The large superfamily of labdane-related diterpenoids is defined by the cyclization of linear geranylgeranyl pyrophosphate (GGPP), catalyzed by copalyl diphosphate synthases (CPSs) to form the basic decalin core, the copalyl diphosphates (CPPs). Here, we used X-ray crystallography and cryo-EM methods to describe different oligomeric structures of a syn-copalyl diphosphate synthase from Oryza sativa (OsCyc1), and provided a cryo-EM structure of OsCyc1D367A mutant in complex with the substrate GGPP. The structure of monomer OsCyc1 consists of an αβγ domain and a catalytic center located between the β and γ domains. OsCyc1 catalyzes GGPP to form syn-CPP, in which new bonds form between C6 and C11, as well as between C10 and C15.

To investigate the substrate binding mode, GGPP was incubated with OsCyc1D367A before cryo-EM sample preparation. We solved the cryo-EM structure of the OsCyc1D367A mutant in complex with substrate GGPP at a resolution of 4 Å. As exemplified by hexamer protomer B, GGPP harbors a continuous and clear density in the active site. We found that while the overall architecture of OsCyc1D367A is similar to that of wild-type OsCyc1, a number of differences exist around the active site, mainly in the loop near residue N405 and helix α7. In the OsCyc1D367A structure, the α7 helix and loops near residues D192 and N405 embrace GGPP more compactly. In the structure of OsCyc1, K233, N405 and K453 interacts with the pyrophosphate, while M194 and E199 are close to the pyrophosphate of GGPP. In OsCyc1D367A structure, the DXDD motif and the conserved basic amino acid, asparagine (N414), are situated at the terminus of the isoprene tail of GGPP. The distance between the d2-oxygen atom in D365 and the carbon-20 atom in the isoprene tail of GGPP is 2.59 Å. However, in the OsCyc1D367A structure, GGPP adopts a linear conformation, possibly reflecting the stage of binding, which might not represent the cyclization state. When we analyzed the structure of OsCyc1D367A, we found that the isoprene tail of GGPP is surrounded by negative and hydrophobic residues.

>[6x]MPVFTASFQCVTLFGQPASAADAQPLLQGQRPFLHLHARRRRPCGPMLISKSPPYPASEETREWEADGQHEHTDELRETTTTMIDGIRTALRSIGEGEISISAYDTSLVALLKRLDGGDGPQFPSTIDWIVQNQLPDGSWGDASFFMMGDRIMSTLACVVALKSWNIHTDKCERGLLFIQENMWRLAHEEEDWMLVGFEIALPSLLDMAKDLDLDIPYDEPALKAIYAERERKLAKIPRDVLHSMPTTLLHSLEGMVDLDWEKLLKLRCLDGSFHCSPASTATAFQQTGDQKCFEYLDGIVKKFNGGVPCIYPLDVYERLWAVDRLTRLGISRHFTSEIEDCLDYIFRNWTPDGLAHTKNCPVKDIADTAMGFRLLRLYGYQVDPCVLKKFEKDGKFFCLHGESNPSSVTPMYNTYRASQLKFPGDDGVLGRAEVFCRSFLQDRRGSNRMKDKWAIAKDIPGEVEYAMDYPWKASLPRIETRLYLDQYGGSGDVWIGKVLHRMTLFCNDLYLKAAKADFSNFQKECRVELNGLRRWYLRSNLEKFGGTDPQTTLMTSYFLASANIFEANRAAERLGWARVALLADAVSSHFRRIGGPKNSTSNLEELISLVPFDDAYSGSLREAWKQWLMAWTAKESSQESIEGDTAILLVRAIEIFGGRHVLTGQRPDLWEYSQLEQLTSSICCKLSRRVLAQENGESTEKVEEIDQQVDLEMQELTRRVLQGCSAINRLTRETFLHVVKSFCYVAYCSPETIDSHIDKVIFQDVIEFHHHHHH>MSLSSGEHEASRVLRERDYRWEGTEEEAYKAEGTHFSGARRQTLVGRPAGQEAPAFETRYFEVEPGGYTTLERHEHTHVVMVVRGHAEVVLDDRVEPLTPLDCVYIAPHAWHQIHATGANEPLGFLCIVDSDRDRPQRP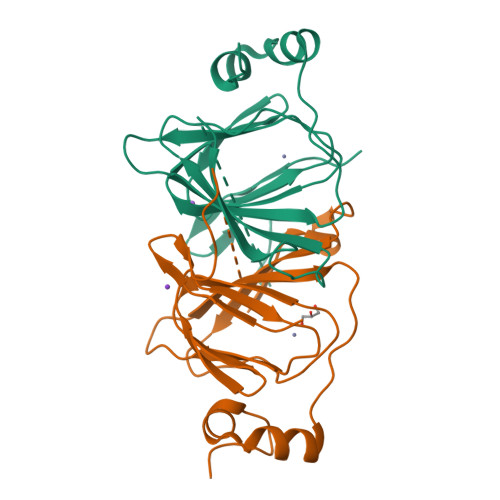DADDLARMCADPAVARRIRTEGHHHHHH[2x]Here, we identify and characterize a unique GlcN kinase from the soil bacterium Streptacidiphilus jiangxiensis, closely related to Streptomyces spp., the classical antibiotic producers. In contrast, from 20 sugars and 4 aminoglycoside antibiotics tested, SjGlcNK only phosphorylated specifically GlcN and displayed vestigial activity with glucose using ATP as a phosphate donor. Determination of the Michaelis constants (Km) for glucose and GlcN suggested that SjGlcNK is better described as a GlcN kinase (EC 2.7.1.8) with a strong preference for using GlcN (Km = 8 ± 1 mM) over glucose (Km > 100 mM) as the substrate. In addition, the structural and biochemical characterization of SjGlcNK provides new insights into the role of these unique GlcN kinases as the missing link for the incorporation of environmental GlcN to the metabolism of GlcNAc in bacteria, an important intermediate in peptidoglycan biosynthesis, glycolysis, and secondary metabolite production.

The crystal structure of SjGlcNK was solved at 1.98-Å resolution and reveals a typical eukaryotic protein kinase fold, consisting of an N-lobe (formed by an N-terminal cap and an intermediate subdomain) and a C-lobe separated by a linker, with a relative arrangement that results in an overall bean shape. The important conserved catalytic motifs, the DFD loop and the catalytic loop, are located in an acidic groove between the two lobes, whereas the P-loop is in the vicinity of this patch. Structural differences between SjGlcNK and mycobacterial maltokinases are mainly found in the N-terminal cap subdomain. The SjGlcNK N-terminal cap is composed of three long antiparallel β-strands (βA-βB-βC) forming a curved β-sheet enclosing α-helices α1 and α2 and by an additional β-strand (βD) perpendicular to strand βB on its concave surface. The intermediate subdomain of SjGlcNK, which is composed of a six-stranded β-sheet (βF-βG-βH-βJ-βI-βE) flanked by two α-helical segments (α3 and α4), is almost identical to that of mycobacterial maltokinases, with a root mean square deviation (RMSD) of 1.7 Å for 80 aligned Cα atoms. A seven-residue linker (residues 187 to 193) connects the intermediate subdomain to the C-terminal lobe (residues 194 to 438), which is composed of two central 4-helical bundles (α5-α6-α10-α11 and α7-α8-α12-α13) and a small two-stranded β-sheet (βK-βL), with an additional helix α9, also present in MtMak, preceding βK and downstream of the catalytic loop. SjGlcNK was crystallized in two different monoclinic (P21) crystal forms, A and B, which differ considerably in the dimensions of the respective unit cells. In consequence, there are two SjGlcNK molecules in the asymmetric unit (AU) of crystal form A, while four monomers are found in the larger AU of crystal form B. In contrast to the structural conservation of the individual subdomains, the relative positions of the N- and C-lobes are strikingly different in the six molecules.

>[2x]MTPNWSELVAAADPALVLPSGERRAEVAVPGPLRLDALLDLGEGHAVGVVRSADAARWTVPLVRDGAGGVRRSRPGDGTAEHLVAALARRGATPDAAFVLEAFTGAAPVTGERGIIVDQTNESVIVGECAVVKWAVRLPAEGEPGSPAAQRIAALARGGFTEMPRPWGLLTLAEGAQPVLLASVVAYLPGALDGWDWAVDDVRRLARGELTMDQALLPAAQLGTLTARMHAALAARGRTPATAADVAAWGVRMREELDEAVASVPGAEGERLKAWAPRIADVYAELDALAGTPLIDVHGDFHVGQILRADGRYAVVDFDGNPVLPADQRAARQPAALDVVGMTASLDHVGRVVVFRTPDVDPAPVRAWIAAAQRSFLDAYRTTLARLDADDLFDDRLLTPLRYAQEVREYLYAVRHLPHWVYVPDLSLTDLLPERLKDKLAAALEHHHHHH1-[(3S,4S)-4-amino-1-(6-phenylpyrimidin-4-yl)pyrrolidin-3-yl]piperidin-2-one 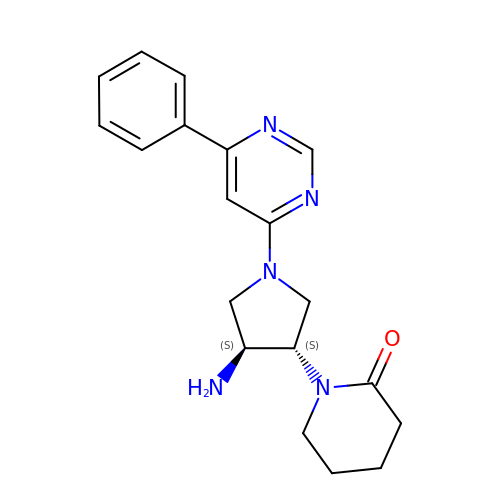| C19 H23 N5 O | FHAABBQZMYZFKY-RDJZCZTQSA-N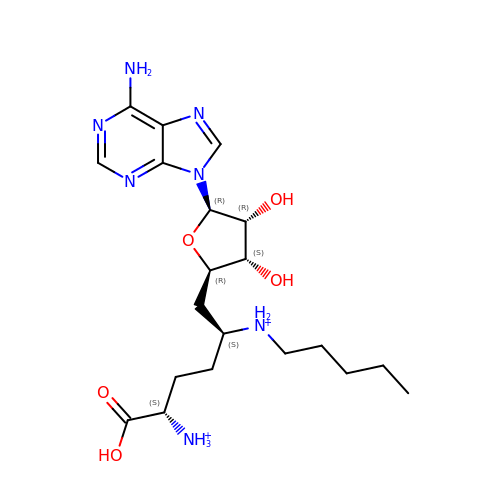[(2~{S},5~{S})-1-[(2~{R},3~{S},4~{R},5~{R})-5-(6-aminopurin-9-yl)-3,4-bis(oxidanyl)oxolan-2-yl]-5-azaniumyl-6-oxidanyl-6-oxidanylidene-hexan-2-yl]-pentyl-azanium | C20 H35 N7 O5 | RFJREUSTWBSNNC-OAVPVUAOSA-P> MQQLTDQSKELDFKSETYKDAYS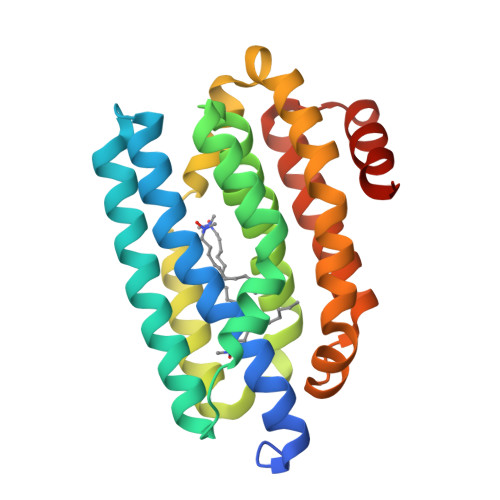RINAIVIEGEQEAHENYITLAQLLPESHDELIRLSKMESRHKKGFEACGRNLAVTPDLQFAKEFFSGLHQNFQTAAAEGKVVTCLLIQSLIIECFAIAAYNIYIPVADDFARKITEGVVKEEYSHLNFGEVWLKEHFAESKAELELANRQNLPIVWKMLNQVEGDAHTMAMEKDALVEDFMIQYGEALSNIGFSTRDIMRLSAYGLIGAPG> MKIEVKDSTMIKPSAETPGGSLWLSNLDLLSPANYHTLSVHF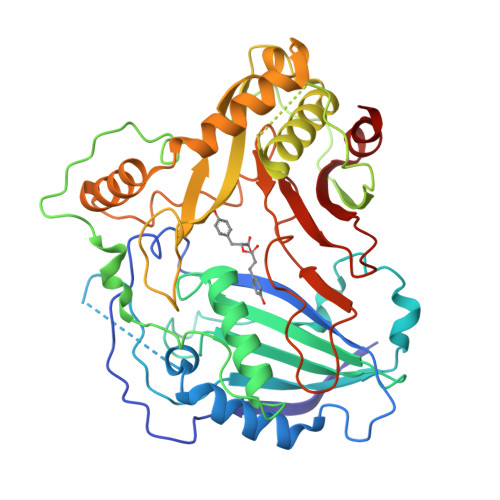YSHDGSDNFFDAAGLKESLSRALVEFYPYAGRLKLNGNRLEIDCNNEGLLLVEAECDGALDELGDFAPRPELNLIPKVDYSRGISTYPLMVFQLTRFKCGGVALGVANEHHLSDGVAALHFINTWAHLSRGAPAPTPLPHFDRSSLSARNPPQPQFSHAEYQPPPTLENPLPHTDIAHSRFKLTRDQLNSLKSKFKTAPADGGAGKSYSTFEVLAGHIWRSVCIARGLPEGQETKLHIPFDGRGRLQLPPGFFGNAIFFATPIATCGEIESNSLNYAVRRVSDGVSRLDEDYLRSSIDFLELQEDISKLAQGAHSFRCPNLWVISWVWLPIYEPDFGWGKAVYMGPWAAPFEGKSYLLPNPEKDGSLFVSITLHKQHMERFEKLFYEI>[4x]GAMQGEVSKAASADSTTEGTPADGFTVLSTKSLFLGQKLQVVQADIASIDSDAVVHPTNTDFYIGGEVGNTLEKKGGKEFVEAVLELRKKNGPLEVAGAAVSAGHGLPAKFV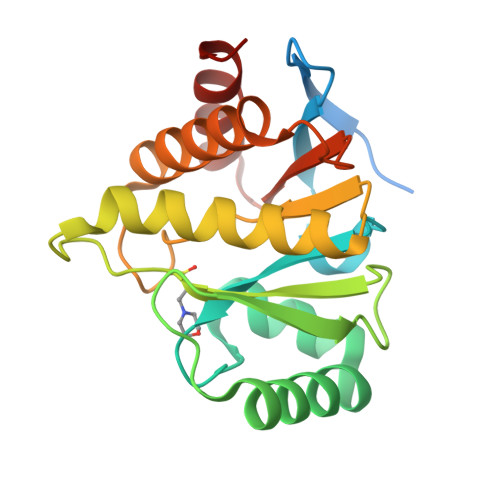IHCNSPVWGADKCEELLEKTVKNCLALADDKKLKSIAFPSIGSGRNGFPKQTAAQLILKAISSYFVSTMSSSIKTVYFVLFDSESIGIYVQEMAKLDAN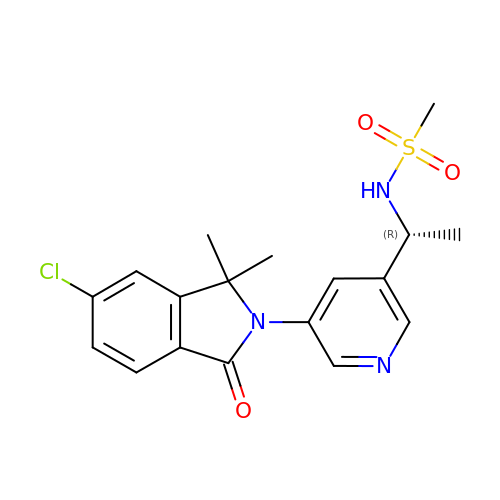~{N}-[(1~{R})-1-[5-(6-chloranyl-1,1-dimethyl-3-oxidanylidene-isoindol-2-yl)pyridin-3-yl]ethyl]methanesulfonamide | C18 H20 Cl N3 O3 S | LXULFFHUCXHBBS-LLVKDONJSA-N(2R)-N-[(4M)-4-(4-amino-2,7-dimethyl-7H-pyrrolo[2,3-d]pyrimidin-5-yl)-3-methylphenyl]-2-hydroxy-2-[3-(trifluoromethyl)phenyl]acetamide | C24 H22 F3 N5 O2 | 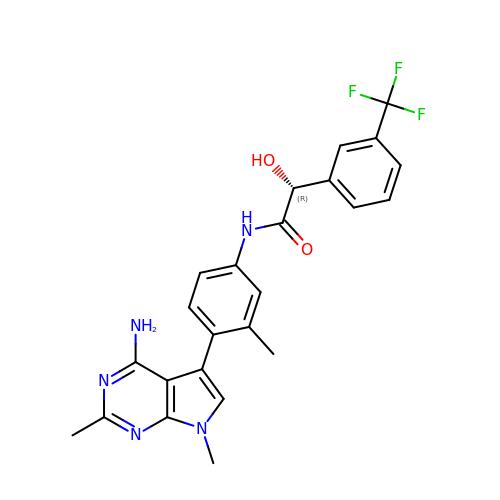GSRBTRZCHOMAAI-HXUWFJFHSA-N>[4x]MAKKTSSKGKLPPGPSPLPVLGNLLQMDRKGLLRSFLRLREKYGDVFTVYLGSRPVVVLCGTDAIREALVDQAEAFSGRGKIAVVDPIFQGYGVIFANGERWRALRRFSLATMRDFGMGKRSVEE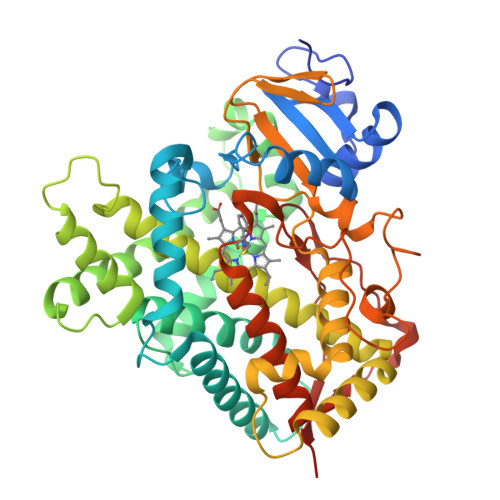RIQEEARCLVEELRKSKGALLDNTLLFHSITSNIICSIVFGKRFDYKDPVFLRLLDLFFQSFSLISSFSSQVFELFSGFLKYFPGTHRQIYRNLQEINTFIGQSVEKHRATLDPSNPRDFIDVYLLRMEKDKSDPSSEFHHQNLILTVLSLFFAGTETTSTTLRYGFLLMLKYPHVTERVQKEIEQVIGSHRPPALDDRAKMPYTDAVIHEIQRLGDLIPFGVPHTVTKDTQFRGYVIPKNTEVFPVLSSALHDPRYFETPNTFNPGHFLDANGALKRNEGFMPFSLGKRICAGEGIARTELFLFFTTILQNFSIASPVPPEDIDLTPRESGVGNVPPSYQIRFLARHHHH> MHNYSYSPGISLLLFILLANTLAIQAVVLPAHQQHLLHNDIADGLDKTALSVSGTQSRWTRSESNPTMRLSQNVKPCKSMDIRNMVSHFNQLENCTVIEGFLLIDLINDASPLNRSFPKLTEVTDYIIIYRVTGLHSLSKIFPNLSVIRGNKLFDGYALVVYSNFDLMDLGLHKLRSITRGGVRIEKNHKLCYDRTIDWLEILAENETQLVVLTENGKEKECRLSKCPGEIRIEEGHDTTAIEGELNASCQLHNNRRLCWNSKLCQTKCPEKCRNNCIDEHTCCSQDCLGGCVIDKNGNESCISCRNVSFNNICMDSCPKG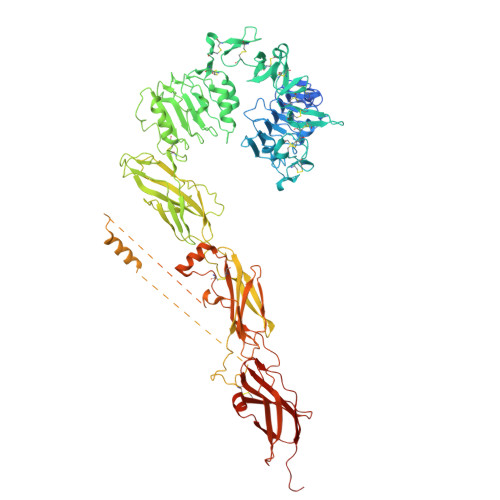YYQFDSRCVTANECITLTKFETNSVYSGIPYNGQCITHCPTGYQKSENKRMCEPCPGGKCDKECSSGLIDSLERAREFHGCTIITGTEPLTISIKRESGAHVMDELKYGLAAVHKIQSSLMVHLTYGLKSLKFFQSLTEISGDPPMDADKYALYVLDNRDLDELWGPNQTVFIRKGGVFFHFNPKLCVSTINQLLPMLASKPKFFEKSDVGADSNGNRGSCGTAVLNVTLQSVGANSAMLNVTTKVEIGEPQKPSNATIVFKDPRAFIGFVFYHMIDPYGNSTKSSDDPCDDRWKVSSPEKSGVMVLSNLIPYTNYSYYVRTMAISSELTNAESDVKNFRTNPGRPSKVTEVVATAISDSKINVTWSYLDKPYGVLTRYFIKAKLINRPTRNNNRDYCTEPLVKAMENDLPATTPTKKISDPLAGDCKCVEGSKKTSSQEYDDRKVQAGMEFENALQNFIFVPNIRKSKNGSSDKSDGAEGAALDSNAIPNGGATNPSRRRRDVALEPELDDVEGSVLLRHVRSITDDTDAFFEKDDENTYKDEEDLSSNKQFYEVFAKELPPNQTHFVFEKLRHFTRYAIFVVACREEIPSEKLRDTSFKKSLCSDYDTVFQTTKRKKFADIVMDLKVDLEHANNTESPVRVRWTPPVDPNGEIVTYEVAYKLQKPDQVEEKKCIPAADFNQTAGYLIKLNEGLYSFRVRANSIAGYGDFTEVEHIKVEPPPSYAKDEVLFQGPSRSAWSHPQFEK>MSHHHHHHSMDIEFVDLEGKTVITSDKAPAAIGPYSQAIKAGNTVYMSGQIPLDPSTMELVEGIEAQITQVFENLKSVAQAAGGSFKDIV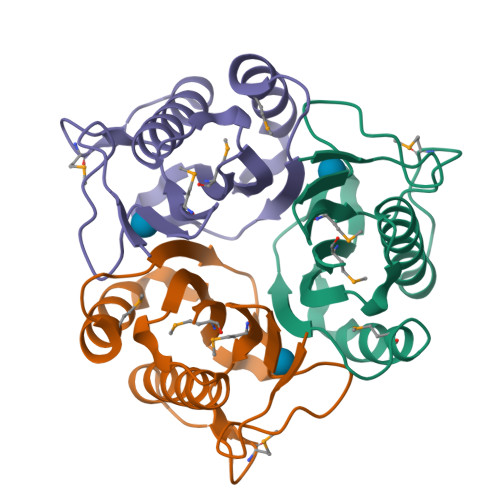KLNIFLTDLGHFAKVNEIMGSYFSQPYPARAAIGVAALPRGAQVEMDAILVIE[3x]> MGNLAGIMHRPDSEMAYVVNEQTVNIRLRTAKDDIVSVELLAGDPYSLRSLPTDEKFYQVPKQMTKIMSDGISDFWQVTVTEPKRRLAYAFLVTDMLGIQKIYSDKGFFKVADADLMDMNFYFRMPFFQTIDQYNAPEWVTDTVWYQIFPERFANGDVSNDPVGTKPWDSTDHPGREDFYGGDLQGILDHLDHLQELGISGIYLNPIFQAPSNHKYDTQDYMTVDPHFGDAKLFKQLVQAAHERGIRVMLDAVFNHIGDKSVQWQDVLKNEQASPYADWFHIHQFPATYTPTDNFEFAADATYDTFDYT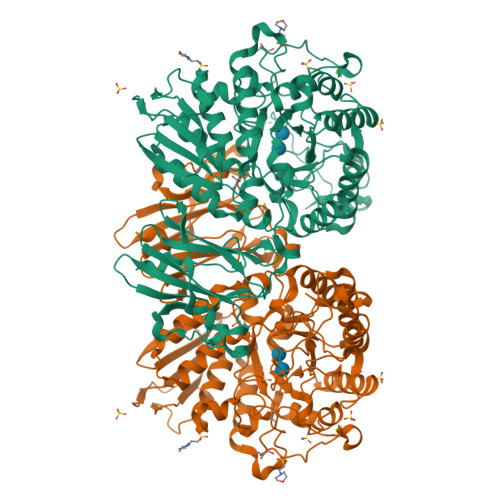PHMPKLNTSNPEVVDYLLNIATYWVKEFDIDAWRLNVANEIDHHFWRKFHDAMMALKPDFYILGEIWHTSQSWLVGDEFTAVMNYSYTGAILQYFLENESADALVQKMSHQLMLYRDATNRMMFNTVDSHDTPRLMTLAHEDKQLAKSILTFTFMQPGVPSIYYGTEYGMTGENDPDDRKPMVWQPELQDHDLYDFMQKLVQVRRQVIAKLSDDKIIFDVIGERQIRLTREDNQTRIVGVFNNGTTDLTVAQPTSILLKTNQSETQLAPNDFMIWTEPVR>MHHHHHHGTNDIIEESAWEALEKSILYYKGRPVGTVAAFDASVEALNYDQCFVRDFVSSALIFLIKGKTDIVRNFLEETLKLQPKDRQLDAYKPGRGLIPASFKVVSDNGEEYLEADFGEHAIARVTPVDSCLWWILLLRAYVVASKDFSLAYQPEFQTGIRLIMEICLANRFDMYPTLLVPDGACMIDRRLGIYGHPLELQVLFYAALRAAREMLICQGNQDVVEAIDNRLPLLCAHIRQHYWIDINRLNAIYRFKSEEYGKAAVNLFNIYVDSIPYYELDKWLPKKGGYLAGNVGPSQLDTRFFALGNLMAIISDLATEEQSQAIMTLIEDRWEDLVGDMPMKICYPALENEEYRIVTGCDPKNIPWSYHNAGSWPVLMWMLAAASVKAGKPYIAGKAIEIAQARLLEDEWPEYYDGKKGRLIGKQARKYQTW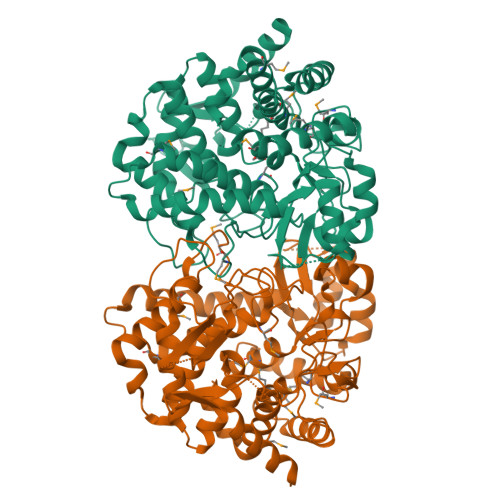TIAGFLLAAELMKNPSLLSLIS[2x]> SSLKPFTYPFPETRFLHAGPNVYKFKIRYGKSIRGEEIENKEVITQELEDSVRVVLGNLDNLQPFATEHFIVFPYK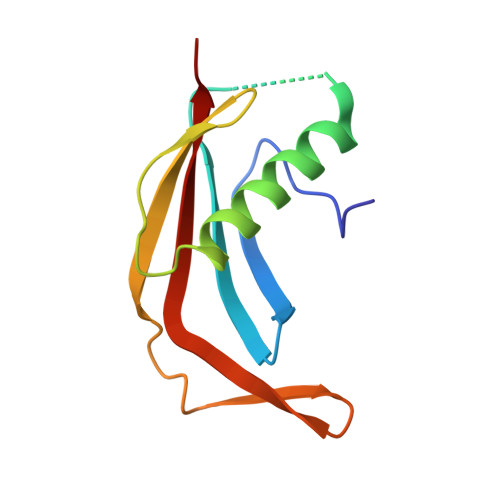SKWERVSHLKFKHGEIILIPYPFVFTLYVEMKW>SNAMAVQLLENWLLKEQEKIQTKYRHLNHISVVEPNILFIGDSIVEYYPLQELFGTSKTIVNRGIRGYQTGLLLENLDAHLYGGAVDKIFLLIGTNDIGKDVPVNEALNNLEAIIQSVARDYPLTEIKLLSILPVNEREEYQQAVYIRSNEKIQNWNQAYQELASAYMQVEFVPVFDCLTDQAGQLKKEYTTDGLHLS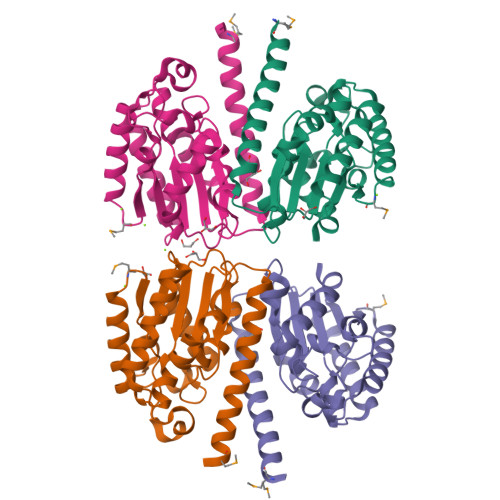IAGYQALSKSLKDYLY[4x]> MK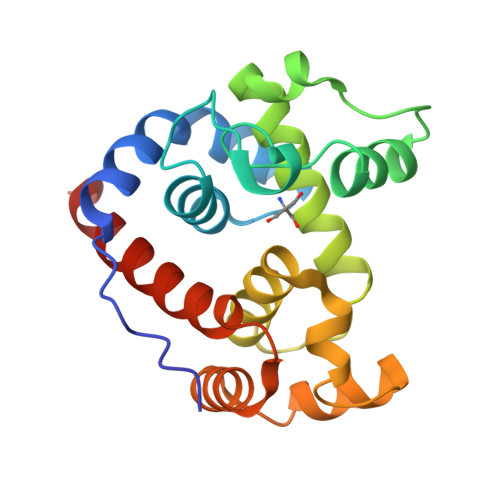HDYTNPPWNAKVPVQRAMQWMPISQKAGAAWGVDPQLITAIIAIESGGNPNAVAKSNAIGLMQLKASTSGRDVYRRMGWSGEPTTSELKNPERNISMGAAYLNILETGPLAGIEDPKVLQYALVVSYANGAGALLRTFSSDRKKAISKINDLDADEFLEHVARNHPAPQAPRYIYKLEQALDAMLEHHHHHH> ASMTPEERAWLAEHPSIRLGVDTSWPPFEFRDEQGRYQGLAAGYVSLLQERKGVSLTPVEPKTWTQVLEQAKDGRLDLLPGIMATPERQEYLSFTRPYLDFPIIILARKNGPMPKRIDELYGLKVAVVDHYAPHELLIAQHPDLTLLPLPSVAAALQALATGQADAFVGDFASSVWNLRQLKLNGLEISGETPYRYQLAMAVPRGQPILAG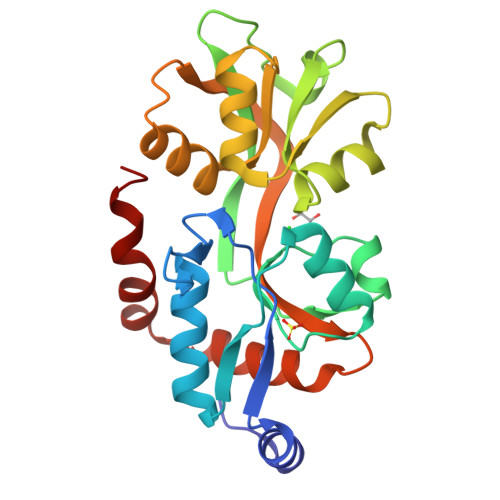IVDKVLADLSAEEIERLQAPWVGGLL> TFSYTLEDHTKQAFGIMNELRLSQQLCDVTLQVKYQDAPAAQFMAHKVVLASSSPVFKAMFTNGLREQGMEVVSIEGIHPKVMERLIEFAYTASISMGEKCVLHVMNGAVMYQIDSVVRACSDFLVQQLDPSNAIGIANFAEQIGCVELHQRAR;> DEKYVNSIWDLLKNAIQEIQRKNNSGLSFEELYRNAYTMVLHKHGEKLYTGLREVVTEHLINKVREDVLNSLNNNFLQTLNQAWNDHQTAMVMIRDILMYMDRVYVQQNNVENVYNLGLIIFRDQVVRYGCIRDHLRQTLLDMIARERKGEVVDRGAIRNACQMLMILGLEG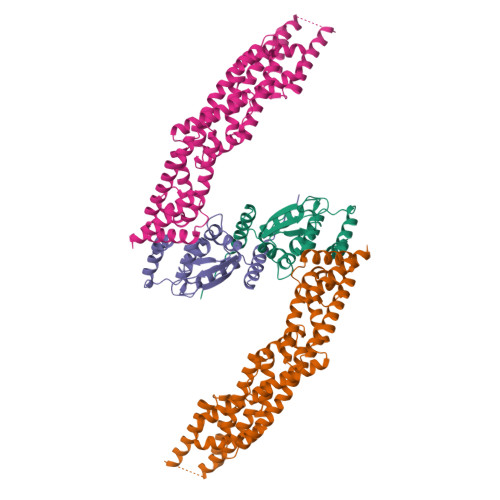RSVYEEDFEAPFLEMSAEFFQMESQKFLAENSASVYIKKVEARINEEIERVMHCLDKSTEEPIVKVVERELISKHMKTIVEMENSGLVHMLKNGKTEDLGCMYKLFSRVPNGLKTMCECMSSYLREQGKALVSEEGEGKNPVDYRQGLDDLKSRFDRFLLESFNNDRLFKQTIAGDFEYFLNLN>GLIYGNYLHLEKVLNAQELQSETKGNKIHDEHLFIITHQAYELWFKQILWELDSVREIFQNGHVRDERNMLKVVSRMHRVSVILKLLVQQFSILETMTALDFNDFREYLSPASGFQSLQFRLLENKIGVLQNMRVPYNRRHYRDNFKGEENELLLKSEQEKTLLELVEAWLERTPGLEPHGFNFWGKLEKNITRGLEEEFIRIQAKEESEEKEEQVAEFQKQKEVLLSLFDEKRHEHLLSKGERRLSYRALQGALMIYFYREEPRFQVPFQLLTSLMDIDSLMTKWRYNHVCMVHRMLGSKAGTGGSSGYHYLRSTVSDRYKVFVDLFNLSTYLIPRHWIPKMNPTIHKFLEHHHHHH[4x]

Tryptophan-2,3-dioxygenase (TDO2) and indoleamine-2,3-dioxygenase (IDO1) are structurally distinct heme enzymes that catalyze the conversion of L-tryptophan to N-formyl-kynurenine, and play important roles in metabolism, inflammation, and tumor immune surveillance. Tryptophan-2,3-dioxygenase (TDO2) and indoleamine-2,3-dioxygenase 1 (IDO1) catalyze the same reaction: the conversion of L-tryptophan (Trp) to N-formyl-kynurenine (NFK). Both enzymes evolved to bind heme for substrate binding and catalysis but are structurally distinct: IDO1 is monomeric, while TDO2 is tetrameric with two independent TDO2 molecules contributing to each of its four active sites. The enzymes can adopt an inactive, heme-free (apo) state or an active, heme-containing (holo) state, with the balance between them varying dynamically according to biological conditions. While apo-TDO2 is catalytically inactive, the term “apo-TDO2 inhibitor” is used to describe compounds that bind to apo-TDO2, compete with heme binding and thus prevent the formation of enzymatically active holo-TDO2.

Two steps were essential for successful co-crystallization of apo-TDO. First, apo-TDO2 was expressed using an E. coli strain that is unable to synthesize heme. Second, the exosite binder AMT was added to apo-TDO2 because of its stabilizing effect as observed in DSF experiments. An exosite that binds both the substrate Trp and its α-methyl analog AMT has been identified previously in holo-TDO224.>MEEECRVLSIQSHVIRGYVGNRAATFPLQVLGFEIDAVNSVQFSNHTGYAHWKGQVLNSDELQELYEGLRLNNMNKYDYVLTGYTRDKSFLAMVVDIVQELKQQNPRLVYVCDPVLGDKWDGEGSMYVPEDLLPVYKEKVVPLADIITPNQFEAELLSGRKIHSQEEALRVMDMLHSMGPDTVVITSSDLPSPQGSNYLIVLGSQRRRNPAGSVVMERIRMDIRKVDAVFVGTGDLFAAMLLAWTHKHPNNLKVACEKTVSTLH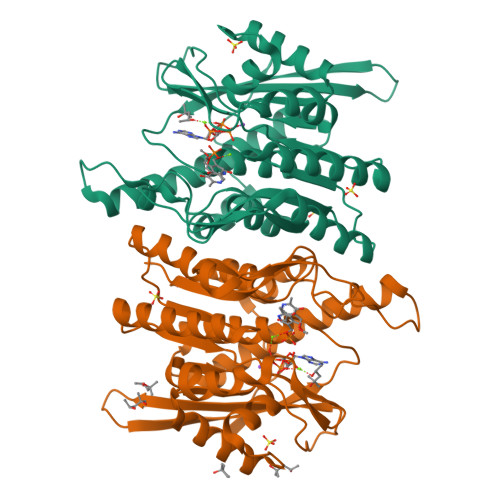HVLQRTIQCAKAQAGEGVRPSPMQLELRMVQSKRDIEDPEIVVQATVL[2x]Sec4p is among the 11 Rab GTPases identified in S. cerevisiae and acts on the surface of membranes to regulate transport between the Golgi apparatus and the plasma membrane. To complete the cycle, the protein is reactivated by switching the guanine nucleotide state from GDP to GTP in a process stimulated by guanine nucleotide exchange factors (GEFs). Therefore, the structural and functional analysis of the mutant Ser29Val of Sec4p offers an opportunity to understand not just the basic differences between Ras GTPase families but also how Sec4p is activated during its GTPase cycle by its GEF Sec2p. Sec2p is a highly efficient exchange factor of Sec4p that stimulates nucleotide exchange by binding to the switch regions of Sec4p and altering its conformation resulting in decreased affinity between Sec4p and nucleotide. In this work we have investigated the nucleotide exchange mechanism of the Rab GTPase Sec4p and how its GEF Sec2p stimulates nucleotide dissociation, making use of the Sec4p mutant S29V corresponding to Gly12 in Ras proteins.

Crystals for the mutant Sec4pV29 were obtained and the structure was solved at 1.9 Å resolution using the wild type Sec4p bound to GDP as a model for molecular replacement. The structure Sec4pV29.GDP contains two molecules in the asymmetric unit (chains A and B). Some of the crystal contacts are made through interactions with zinc atoms that are coordinated by Asp43 and Asp166 from molecule B, and His121 from molecule A. Besides the presence of the mutation S29V, the P-loop region from Sec4pV29.GDP and Sec4pwt.GDP superpose almost perfectly. Furthermore, all the interactions between protein and nucleotide are conserved between the two structures. The switch I region is disordered in the molecule A and ordered in molecule B. The SWI of molecule B adopts a different conformation from that observed on the Sec4pwt.GDP structure. However, this new conformation is held in place by interactions with symmetric related molecules and is probably an artifact of crystal packing. One of the most intriguing observations made for the Sec4pwt.GDP was the interaction between the Arg81 of the SWII and the Ser29 of the P-loop. The side chain of the residue Arg81 forms a 2.8 Å length hydrogen bond with the side chain of the Ser29 residue. This interaction is not observed in the Sec4pV29.GDP structure. The structure of Sec4pV29.GDP presents a very similar fold to the wild type protein indicating that the decrease in the intrinsic nucleotide dissociation rate is not due to large conformational changes. The difference in nucleotide dissociation rate is most likely explained by changes in the protein-nucleotide environment created by the hydrophobic side chain of the Val29.

>[2x]SSIMKILLIGDVGVGKSCLLVRFVEDKFNPSFITTIGIDFKIKTVDINGKKVKLQLWDTAGQERFRTITTAYYRGAMGIILVYDVTDERTFTNIKQWFKTVNEHANDEAQLLLVGNKSDMETRVVTADQGEALAKELGIPFIESSAKNDDNVNEIFFTLAKLIQEKIDSN Import of proteins into peroxisomes depends on PEX5, PEX13 and PEX14. By combining biochemical methods and structural biology, we show that the C-terminal SH3 domain of PEX13 mediates intramolecular interactions with a proximal FxxxF motif. The SH3 domain also binds WxxxF peptide motifs in the import receptor PEX5, demonstrating evolutionary conservation of such interactions from yeast to human. Strikingly, intramolecular interaction of the PEX13 FxxxF motif regulates binding of PEX5 WxxxF/Y motifs to the PEX13 SH3 domain.

Our results demonstrate that the PEX13 SH3 domain indeed binds to WxxxF/Y motifs in PEX5 and that this interaction is conserved from yeast to human. Notably, the PEX5 WxxxF and FxxxF binding sites overlap and are thus competitive. The PEX5 W4 motif was identified as the strongest binder followed by W2 and W3. Of note, amongst the eight motifs in PEX5, W4 shows the highest relative binding affinity for PEX13 SH3 and the weakest interaction with the PEX14 NTD. To investigate the structural basis for the PEX5 W4 / PEX13 SH3 interaction, we determined the crystal structure of a PEX13 SH3 GS W4 chimera. In contrast to the PEX13 FxxxF motif, the binding interface is limited to the core motif driven by hydrophobic interactions and few hydrogen bonds from R183, Y185, and Y188 to the backbone or K304 sidechain. Nevertheless, polar backbone interactions involving G335 and K336 and coordination from K304 seem important since they are conserved from PEX13 FxxxF to PEX5 W4 (colored lines). Our crystal structure of PEX13 SH3 with the W4 motif reports high-resolution details for this non-canonical binding interface of an SH3 domain fold.

>[2x]VTDSINWASGEDDHVVARAEYDFAAVSEEEISFRAGDMLNLALKEQQPKVRGWLLASLDGQTTGLIPANYVKILGKRKGRKTVESSGGGGSTATDRWYDEYHPEE> MSHQERLQSKSLHLSPQEQSASYQDRRQSWRRASMKETNRRKSLHPIHQGITELSRSISVDLAESKRLGCLLLSSFQFSIQKLEPFLRDTKGFSLESFRAKASSLSEELKHFADGLETDGTLQKCFEDSNGKAS;> GPLGSSATPREDFRVRCTSKRAVTEMLQLCGRFVQKLGDALPEEIREPALRDAQWTFESAVQENISINGQAWQEAS

Kinetochores, multisubunit protein assemblies, connect chromosomes to spindle microtubules to promote chromosome segregation. The 10-subunit KMN assembly (comprising KNL1, MIS12, and NDC80 complexes, designated KNL1C, MIS12C, and NDC80C) binds microtubules and regulates mitotic checkpoint function through NDC80C and KNL1C, respectively. The 10-subunit KMN assembly consists of three complexes, the 4-subunit MIS12 complex (MIS12C), the 2-subunit KNL1 complex (KNL1C), and the 4-subunit NDC80 complex (NDC80C) (Bharadwaj et al., 2004, Cheeseman et al., 2004, De Wulf et al., 2003, Desai et al., 2003, Kline et al., 2006, McCleland et al., 2003, Nekrasov et al., 2003, Obuse et al., 2004, Pinsky et al., 2003, Westermann et al., 2003, Wigge and Kilmartin, 2001). Human MIS12C (also known as MIND complex or Mtw1 complex in Saccharomyces cerevisiae) contains the MIS12, PMF1, NSL1, and DSN1 subunits (synonyms are reported in Table S1A). Finally, MIS12C is a binding hub that connects the other two KMN complexes to CCAN through an interaction with CENP-C (Gascoigne et al., 2011, Hori et al., 2013, Hornung et al., 2011, Hornung et al., 2014, Liu et al., 2016, Maskell et al., 2010, Petrovic et al., 2010, Przewloka et al., 2011, Screpanti et al., 2011).

In addition, we report the crystal structure of the isolated Head2 domain determined at 2.0 Å. The buried surface areas (Collaborative Computational Project, Number 4, 1994) for the MIS12:PMF1 and DSN1:NSL1 pairs (4,209 and 3,575 Å2) are much larger than those of the four other interfaces, which range between 465 and 1,905 Å2. Both subcomplexes start with N-terminal helical hairpins that interact in four-helix bundles (defined here as “Head1” and “Head2” domains for the MIS12:PMF1 and DSN1:NSL1 subcomplexes, respectively) and progress into a “stalk” region. The helical connector joins Head2 to the stalk, but Head2 itself is less restrained, as its linkage to the helical connector is extended and apparently flexible. We speculated that the detachment of Head2 from the core of the MIS12C might, at least in part, explain our difficulties in obtaining well-ordered crystals of MIS12C. Thus, Head1 is necessary, but not sufficient, for high-affinity binding of MIS12C to CENP-C. As expected, we saw no binding of Head2 to CENP-C. Thus, Head2 and the segments that precede it (also deleted in the MIS12CΔHead2 construct) are not required for CENP-C binding.>MASSMRSLFSDHGKYVESFRRFLNHSTEHQCMQEFMDKKLPGIIGRIGDTKSEIKILSIGGGAGEIDLQILSKVQAQYPGVCINNEVVEPSAEQIAKYKELVAKTSNLENVKFAWHKETSSEYQSRMLEKKELQKWDFIHMIQMLYY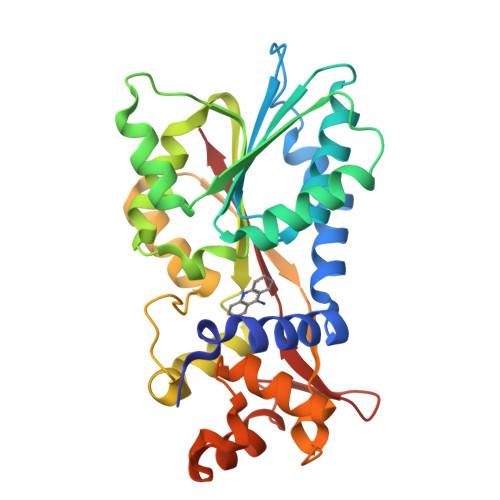VKDIPATLKFFHSLLGTNAKMLIIVVSGSSGWDKLWKKYGSRFPQDDLCQYITSDDLTQMLDNLGLKYECYDLLSTMDISDCFIDGNENGDLLWDFLTETCNFNATAPPDLRAELGKDLQEPEFSAKKEGKVLFNNTLSFIVIEA[2x]>[2x]MVEFKILEKRPDSIKFIVSGVDVPFANALRRTILSEVPTFAVDEVEFLENDSALFDEIIAHRLAMIPLTTPHERFSLDALELDDYTVTLSLEAEGPGMVYSGDLKSSDGDVKPANPNIPIVKLAEGQRLTFNAYARLGRG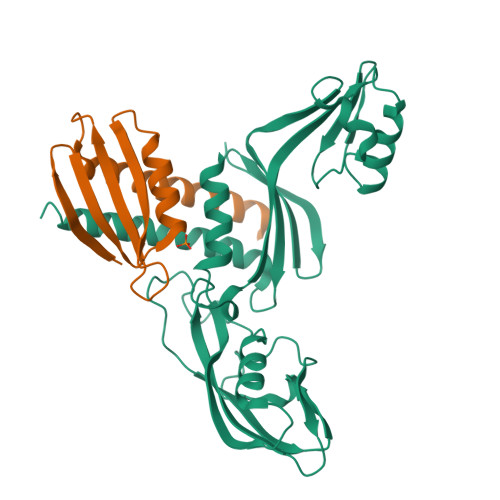KDHAKWQPGFVYYKYLTKIHVSKDVPDWEELKELAERRGLPVEESDEEIVITTIKAFYLPRKFEEHMGKGIREEIVPGSFVFTVETNGELPVEEIVSIALKILMRKSDRFINELHKLAD;>[2x]MRIEVIRREENLLEFYLEGEDHTFANLLTETLHENEHVTFAGYTIEHPITMARKPRFKVVTDGKITPEKALEEAAQKIFDRAREVLEAWKAAIE>MAHHHHHHMSQLSTIIEQAFEDRANFTAADCPSEIRQAVEEAIAGLDNGTLRVAEKINGEWVVHQWLKKAVLLSFKLNDNKPIESCDLRFYDKVETKFSGWTEEQFKAAGVRVVPPAVARRGSFQAKNVVLMPSYVNIGAYVDEGTMVDTWATVGSCAQIGKNVHLSGGVGIGG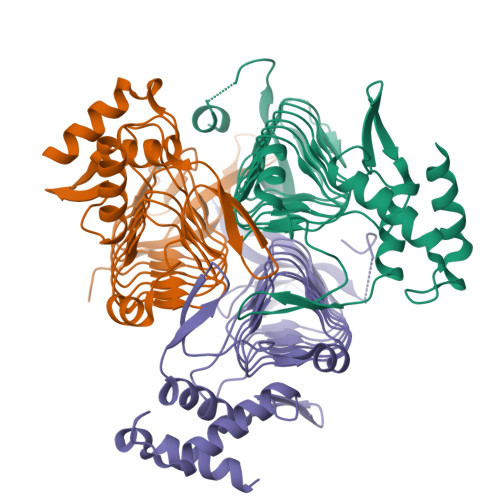VLEPLQANPTIIEDNCFIGARSEIVEGVIVEEGSVISMGVYIGQSTRIYDRETGEIHYGRVPAGSVVVPGNLPSADGKYSLYAAIIVKKVDAQTRAKTSLNDLLRAD[3x]>MTPESVMMMGTEAMKVALALAAPLLLVALITGLIISILQAATQINEMTLSFIPKIVAVFIAIIVAGPWMLNLLLDYVRTLFSNLPYIIG[4x];> MIQVTSEQWLYWLHLYFWPLLRVLALISTAPILSERAIPKRVKLGLGIMITLVIAPSLPANDTPLFSIAALWLAMQQILIGIALGFTMQFAFAAVRTAGEFIGLQMGLSFATFVDPGSHLNMPVLARIMDMLAMLLFLTFNGHLWLISLLVDTFHTLPIGSNPVNSNAFMALARAGGLIFLNGLMLALPVITLLLTLNLALGLLNRMAPQLSIFVIGFPLTLTVGIMLMAALMPLIAPFCEHLFSEIFNLLADIVSEMPINNNP;>MRRLLFLSLAGLWLFSPAAAAQLPGLISQPLAGGGQSWSLSVQTLVFITSLTFLPAILLMMTSFTRIIIVFGLLRNALGTPSAPPNQVLLGLALFLTFFIMSPVIDKIYVDAYQPFSEQKISMQEALDKGAQPLRAFMLRQTREADLALFARLANSGPLQGPEAVPMRILLPAYVTSELKTAFQIGFTIFIPFLIIDLVIASVLMALGMMMVPPATIALPFKLMLFVLVDGWQLLMGSLAQSFYS[5x];>[6x]MAAIQGIEGVISQLQATAMAARGQDTHSQSTVSFAGQLHAALDRISDRQAAARVQAEKFTLGEPGIALNDVMADMQKASVSMQMGIQVRNKLVAAYQEVMSMQV;>MLDRLDAALRFQQEALNLRAQRQEILAANIANADTPGYQARDIDFASELKKVMVRGREETGGVALTLTSSHHIPAQAVSSPAVDLLYRVPDQPSLDGNTVDMDRERTQFADNSLKYQMGLTVLGSQLKGMMNVLQGGN[5x];>[6x]MALLNIFDIAGSALAAQSKRLNVAASNLANADSVTGPDGQPYRAKQVVFQVDAAPGQATGGVKVASVIESQAPEKLVYEPGNPLADANGYVKMPNVDVVGEMVNTMSASRSYQANIEVLNTVKSMMLKTLTLGQ;>MSATASTATQPKPLEWLNRLRANPRIPLIVAGSAAVAIVVAMVLWAKTPDYRTLFSNLSDQDGGAIVAQLTQMNIPYRFANGSGAIEVPADKVHELRLRLAQQGLPKGGAVGFELLDQEKFGISQFSEQVNYQRALEGELARTIETLGPVKSARVHLAMPKPSLFVREQKSPSASVTVTLEPGRALDEGQISAVVHLVSSAVAGLPPGNVTLVDQSGHLLTQSNTSGRDLNDAQLKFANDVESRIQRRIEAILSPIVGNGNVHAQVTAQLDFANKEQTEEHYSPNGDASKATLRSRQLNISEQVGAGYPGGVPGALSNQPAPPNEAPIATPPTNQQNAQNTPQTSTSTNSNSAGPRSTQRNETSNYEVDRTIRHTKMNVGDIERLSVAVVVNYKTLADGKPLPLTADQMKQIEDLTREAMGFSDKRGDTLNVVNSPFSAVDNTGGELPFWQQQSFIDQLLAAGRWLLVLVVAWILWRKAVRPQLTRRVEEAKAAQEQAQVRQETEEAVEVRLSKDEQLQQRRANQRLGAEVMSQRIREMSDNDPRVVALVIRQWMSNDHE[11x];>[5x]MDHAIYTAMGAASQTLNQQAVTASNLANASTPGFRAQLNALRAVPVDGLSLATRTLVTASTPGADMTPGQLDYTSRPLDVALQQDGWLVVQAADGAEGYTRNGNIQVGPTGQLTIQGHPVIGEGGPITVPEGSEITIAADGTISALNPGDPPNTVAPVGRLKLVKAEGNEVQRSDDGLFRLTAEAQAERGAVLAADPSIRIMSGVLEGSNVKPVEAMTDMIANARRFEMQMKVITSVDENEGRANQLLSMS

The bacterial flagellar motor is a huge bidirectional rotary nanomachine that drives rotation of the flagellum for bacterial motility. The cytoplasmic C ring of the flagellar motor functions as the switch complex for the rotational direction switching from counterclockwise to clockwise. The basal body is made up of the LP ring, MS ring, C ring, rod and export apparatus. Here, we present two high-resolution cryo-electron microscopy structures of the C ring-containing flagellar basal body–hook complex from Salmonella Typhimurium, which are in the default counterclockwise state and in a constitutively active CheY mutant-induced clockwise state, respectively.

To obtain the C ring-containing basal body–hook complex in the CW state, we constructed the constitutively active double mutant D13K/Y106W of CheY (hereafter referred to as CheY**), which can mimic CheY-P to tightly bind to the C ring and lock the rotational direction of the motor in the CW state. The density maps of the LP ring, MS ring, rod, hook, and export apparatus in the CW state were locally reconstructed to the higher resolutions ranging from 2.8 Å to 3.8 Å. Although the structures of the LP ring, MS ring, rod, hook, and export apparatus in the CW state are highly similar to those of these components in the CCW state, the protomers of the C ring in the CW state notably undergo inclination and compaction, suggesting that the binding of CheY** induces significant conformational changes of the C ring for rotational switching. In the intact C ring-containing basal body–hook complexes, there is one more peptide loop L3, which consists of the residues G310–P322 of FliF and is also extended from the β-collar region of the MS ring, bound in a hydrophobic groove that is formed by the α2–α3 linking loop of FliE6 with the D0 and DC domains of FlgC1 and FlgC6 on the surface of the rod.2-[(chloroacetyl)amino]-5-[(E)-(4-sulfophenyl)diazenyl]benzenesulfonic acid | C14 H12 Cl N3 O7 S2 | 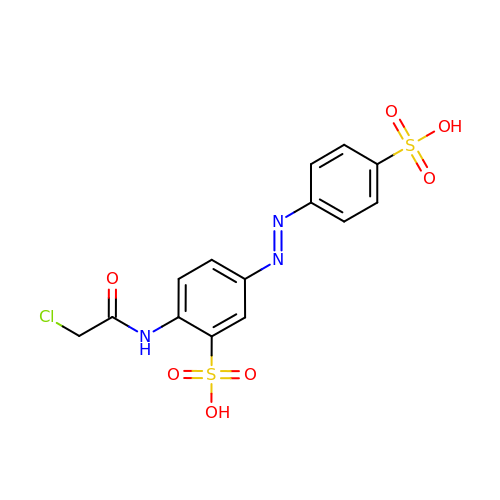VKZZMWQUZNYGMS-ISLYRVAYSA-N> GHMSVYHHILLAVDFSSEDSQVVQKVRNLASQIGARLSLIHVLDNIPMPDTPYGTAIPLDTETTYDAMLDVEKQKLSQIGNTLGIDPAHRWLVWGEPREEIIRIAEQENVDLIVVGSHGRHGLALLLGSTANSVLHYAKCDVLAVRLRDD

Universal stress proteins (USP) are widely spread proteins in nature. In stress conditions such as heat shock, nutrient starvation, the presence of oxidants, uncouplers, DNA-damaging agents, or other stress agents which may arrest cell growth, USP constitute a natural biological defense mechanism. Under stress, USPs are overproduced and through a variety of mechanisms aid the organism in surviving in such uncomfortable conditions. Here, we present the structures of both apo- and cofactor-bound forms of an euryarchaeal USP AF0826 from A. fulgidus and a bacterial USP NE1028 from N. europaea.

The best-studied USP protein MJ0577-ATP from M. janashii contains a typical ATP-binding motif, which is composed of the following residues: G127-SH-G130-(9X)-G140S141V142 (where the superscripts indicate the position of each residue in the sequence). This motif corresponds to the following residues in NE1028: G114-SH-G117-(8X)-G126S127T128, suggesting that the N. europea USP may be able to bind ATP. Our structure of NE1028–AMP confirms that the protein can bind at least one molecule of ATP analog per monomer. In the NE1028–AMP structure, a conserved stretch of nonpolar residues (as visible on summarizing multiple sequence alignment—Fig. 8), followed by D14 and also strongly conserved S/T residues and V42, form contacts with the adenine ring. The first three residues from the conserved motif (G116-SH-) contacts ribose and the T130 residue binds the phosphates. As a result, we obtained the structure of AF0826 with dAMP bound in the vicinity of the ATP-binding motif. All of the residues binding dAMP in AF0826 are analogs of the residues binding AMP in the NE1028 structure, and interact with the ligand in very similar ways, as shown in Fig. 4B and D. Where hydroxyl groups are interacting with G and A (AF0826: G103, A9; NE1028: G114, A10) and adenine ring is positioned by either V or S (S40 and V40, respectively).> MVMSKYQSVNPYTNEAFASYDNPTSKQIDEAINLAHALYKKWRHEEPASRAEILHDIANALKEHEDELAKMMTLEMGKLLSESKEEVELCVSICNYYADHGPEMLKPTKLNSDLGNAY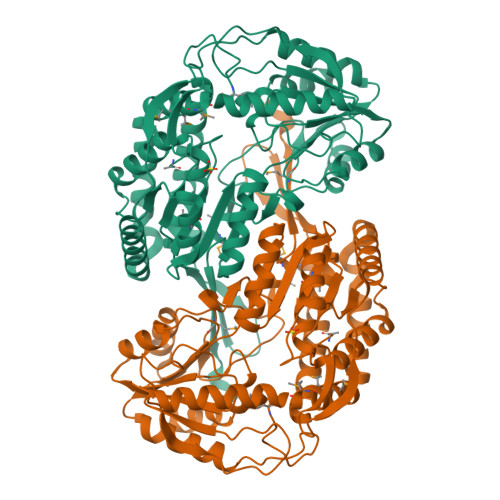YLKQSTGVIMACEPWNFPLYQVIRVFAPNFIVGNPILLKHAHNVPGSAALTAKIIKRAGAPEGSLINLYPSYDQLADIIADPRIQGVALTGSERGGSAVAEAAGKNLKKSTMELGGNDAFIVLDDADPQVLRNVLNDARTYNDGQVCTSSKRIIVEKSRYDEVLHELKNVFSNLKAGDPLEADTTLPPMNSEKAKEKLEAQVKEAIDAGAKVFYQYPEIDSKGAFFRPTILTDIAKDNPVFDKEVFGPIAEVFVVEDDNAAIQLANDSSYGLGSSVIGSDIDRAKKVSAQIETGMTVINGRWITSGELPFGGIKKSGYGRELSGLGLMAFVNEHLVIDVTKNNQAENLYFQSHHHHHHWSHPQFEK1-[(2,4-dichlorophenyl)methyl]pyrazole-3,5-dicarboxylic acid | C12 H8 Cl2 N2 O4 | 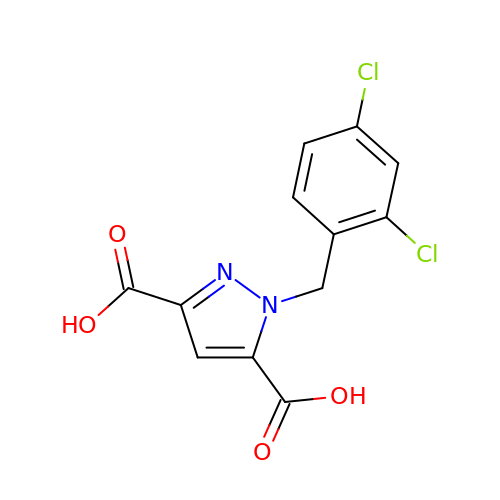FIUGGBBCGGFVRL-UHFFFAOYSA-N> GSFTMDHYLDIRLRPDPEFPPAQLMSVLFGKLHQALVAQGGDRIGVSFP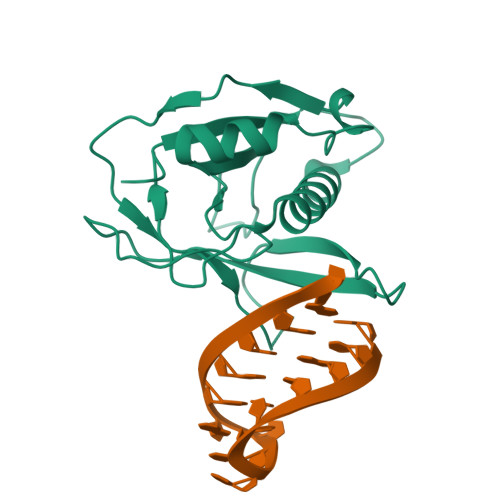DLDESRSRLGERLRIHASADDLRALLARPWLEGLRDHLQFGEPAVVPHPTPYRQVSRVQAKSNPERLRRRLMRRHDLSEEEARKRIPDTVARALDLPFVTLRAQSTGQHFRLFIRHGPLQVTAEEGGFTCYGLSKGGFVPWF>MSQIPASEQETLVRPKPLLLKLLKSVGAQKDTYTMKEVLFYLGQYIM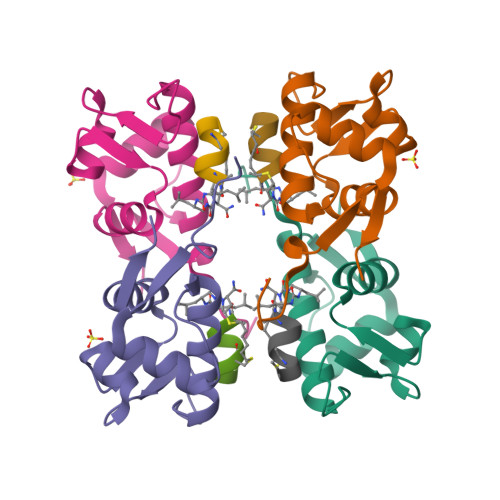TKRLYDEKQQHIVYCSNDLLGDLFGVPSFSVKEHRKIYTMIYRNLVVVN[4x]>TNLLPNIKEDKMLTLRREIKSPSKSALDSFTLIMQTYNRTDLLLRLLNHYQAVPSLHKVIVVWNNVGEKGPEELWNSLGPHPIPVIFKPQTANKMRNRLQVFPEVETNAVLMVDDDTLISAQDLVFAFSIWQQFPDQIIGFVPRKHVSTSSGIYSYGGFELQTPGPGNGDQYSMVLIGASFFNSKYLELFQKQPAAVHALIDETQNCDDIAMNFLVTRHTGKPSGIFVKPI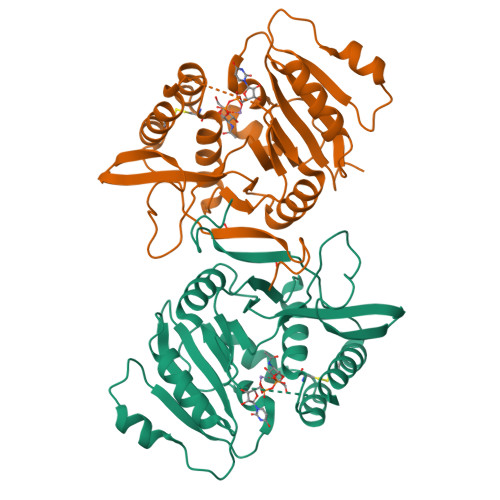NMVNLEKETNGYSGMWHRAEHFLQRSYCINKLVNIYDGMPLKYSNIMISQFGFPYANHKSKM[2x]3-(1-methylpiperidinium-1-yl)propane-1-sulfonate | C9 H19 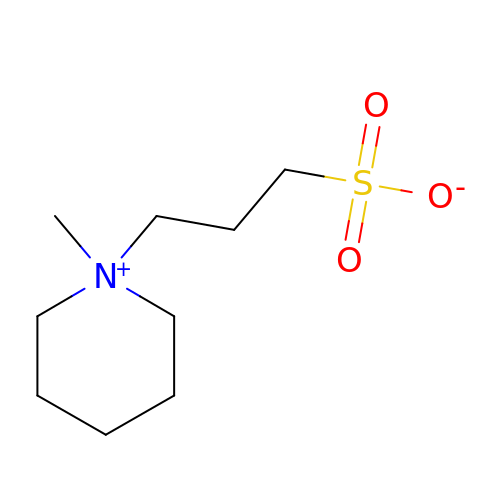N O3 S | DQNQWAVIDNVATL-UHFFFAOYSA-N5-(7-(4-(4,5-DIHYDRO-2-OXAZOLYL)PHENOXY)HEPTYL)-3-METHYL ISOXAZOLE | C20 H26 N2 O3 | 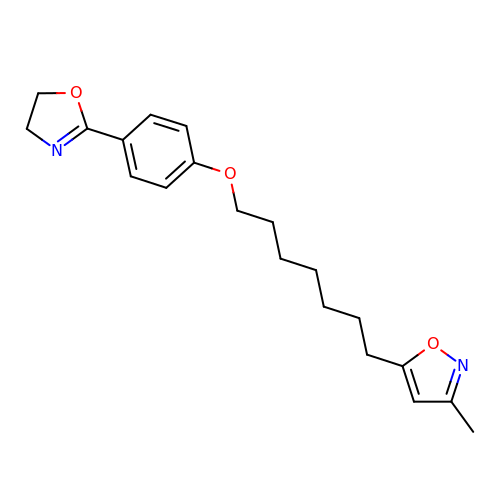FKLJPTJMIBLJAV-UHFFFAOYSA-N>[2x]GSMAQQMAFDISVNASKTINALVYFSTQQNKLVIRNEVNDT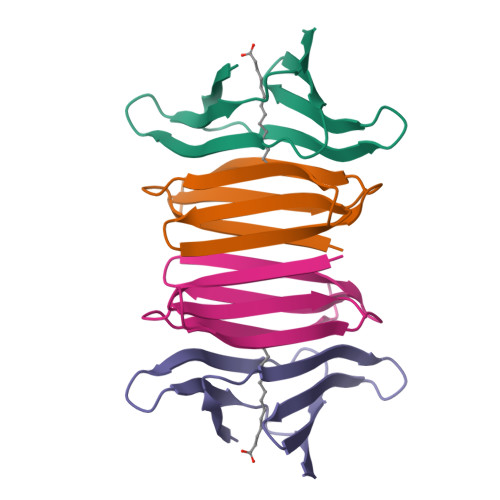HYTVEFDRDKVVDTFISYNRHNDTIEIRGVLPEETNIGCAVNTPVSMT>MEGGGKPNSSSNSRDDGNSVFPAKASATGAGPAAAEKRLGTPPGGGGAGAKEHGNSVCFKVDGGGGGGGGGGGGEEPAGGFEDAEGPRRQYGFMQRQFTSMLQPGVNKFSLRMFGSQKAVEKEQERVKTAGFWIIHPYSDFRFYWDLIMLIMMVGNLVIIPVGITFFTEQTTTPWIIFNVASDTVCLLDLIMNFRTGTVNEDSSEIILDPKVIKMNYLKSWFVVDFISSIPVDYIFLIVEKGMDSEVYKTARALRIVRFTKILCLLRLLRLSRLIRYIHQWEEIFHMTYDLASAVVRIFNLIGMMLLLCHWDGCLQFLVPLLQDFPPDCWVSLNEMVNDSWGKQYSYALFKAMSHMLCIGYGAQAPVSMSDLWITMLSMIVGATCYAMFVGHATALIQSLDSSRRQYQEKYKQVEQYMSFHKLPADMRQKIHDYYEHRYQGKIFDEENILNELNDPLREEIVNFNCRKLVATMPLFANADPNFVTAMLSKLRFEVFQPGDYIIREGAVGKKMYFIQHGVAGVITKSSKEMKLTDGSYFGEICLLTKGRRTASVRADTYCRLY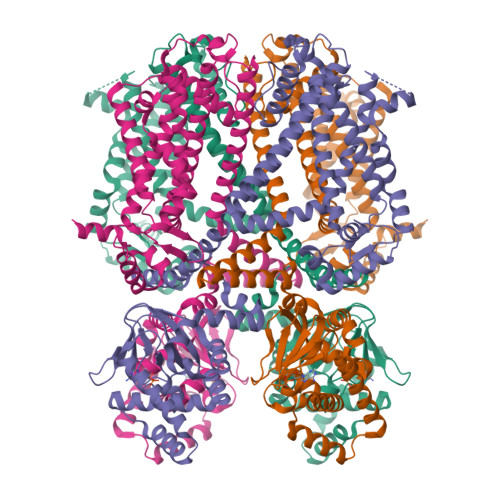SLSVDNFNEVLEEYPMMRRAFETVAIDRLDRIGKKNSILLQKFQKDLNTGVFNNQENEILKQIVKHDREMVQAALPRESSSVLNTDPDAEKPRFASNL[4x]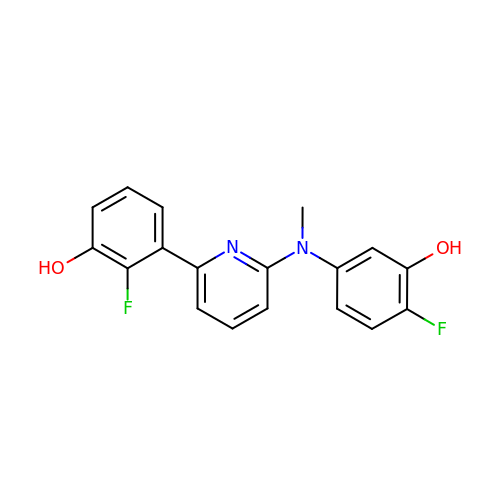2-fluoranyl-3-[6-[(4-fluoranyl-3-oxidanyl-phenyl)-methyl-amino]pyridin-2-yl]phenol | C18 H14 F2 N2 O2 | TZILIAOKSRIZHK-UHFFFAOYSA-N> MAFNYTPLTETQKLKDMYPKVNDIGNFLKTEVNLSDVKQISQPDFNNILASIPDSGNYYVTNSKGAPSGEATAGFVRLDKRNVNYYKIYYSPYSSNKMYIKTYANGTVYDWISFKLDEGSLYNEGNTLNVKELTESTTQYATLVNPPKENLNTGWVNYKESKNGVSSLVEFNPVNSTSTFKMIRKLPVQEQKPNLLKDSLFVYPETSYSNIKTDNWDTPPFWGYSSNSGRSGVRFRGENTVQIDDGSDTYPSVVSNRFKMGKELSVGDTVTVSVYAKINDPALLKDNLVYFELAGYDTVDDTSKNPYTGGRREITASEITT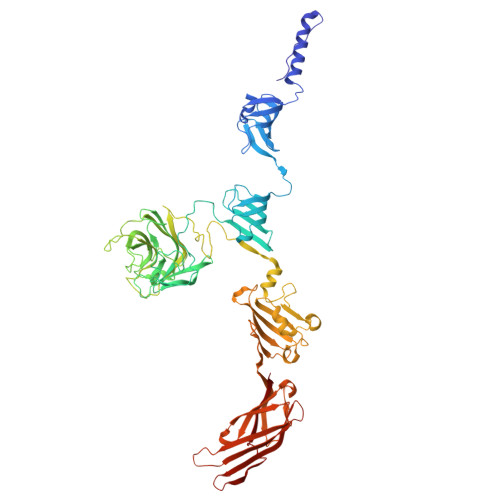EWKKYSFTFTIPENTIGASGVKVNYVSLLLRMNCSSSKGNGAVVYYALPKLEKSSKVTPFITHENDVRKYDEIWSNWQEVISKDELKGHSPVDIEYNDYFKYQWWKSEVNEKSLKDLAMTVPQGYHTFYCQGSIAGTPKGRSIRGTIQVDYDKCDPYRANKFVKLLFTDTEGIPYTLYYGGYNQGWKPLKQSETSTLLWKGTLDFGSTEAVNLNDSLDNYDLIEVTYWTRSAGHFSTKRLDIKNTSNLLYIRDFNISNDSTGSSVDFFEGYCTFPTRTSVQPGMVKSITLDGSTNTTKVASWNEKERIKVYNIMGINRG>[2x]MKIGIIGAMQQEV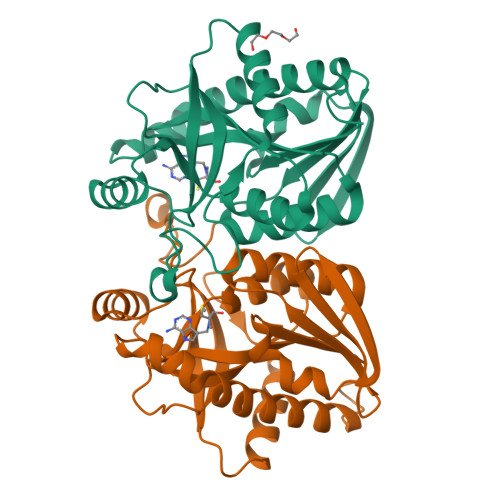AILKDLIEDVQEVNQAGCTFYSGQIQGVDVVLLQSGIGKVSAALGTALLISQYAPDVVINTGSAGGFDASLNVGDVVISSEVRHHDADVTAFGYEIGQMPGQPAAFKADEKLMTVAEQALAQLPNTHAVRGLICTGDAFICTAEGQQFIRQHFPSVVAVEMEASAIAQTCHQFKVPFVVVRAISDVADKESPLSFEEFLPLAAKSSSAMVLKMVELLKENLYFQGHHHHHH Replication of the ∼30 kb-long coronavirus genome is mediated by a complex of non-structural proteins (NSP), in which NSP7 and NSP8 play a critical role in regulating the RNA-dependent RNA polymerase (RdRP) activity of NSP12. The central unit of the replication machinery is NSP12, which is responsible for the RNA-dependent RNA polymerase (RdRP) activity. In addition, NSP7 and NSP8, with molecular weights of ∼9 and ∼22 kDa, respectively, serve to promote the replication processivity of NSP12 (5,6). We report the crystal structure of the complex between NSP7 and NSP8 of SARS-CoV-2, revealing a 2:2 heterotetrameric form.

Next, we crystalized the NSP7–NSP8 complex and solved the crystal structure at 2.7 Å resolution. The crystal structure of the NSP7-NSP8 complex belongs to the space group P21, with each asymmetric unit containing two NSP7 and NSP8 molecules. Despite the fact that full-length NSP7 and NSP8 proteins were prepared for crystallization, we were only able to trace the electron density for the C-terminal domain of NSP8 spanning from residues E77 to S193, with the N-terminal portion most likely proteolytically cleaved during crystallization. On the other hand, we were able to trace the entire NSP7 molecule except for residues L83-Q84 at its C-terminus. Analysis of the structure of the NSP7–NSP8 complex reveals a 2:2 NSP7–NSP8 tetrameric complex, formed by two closely-packed NSP7–NSP8 dimers. As previously observed for the NSP7–NSP8–NSP12 complex, NSP8 is comprised of an N-terminal domain, albeit with only two α-helices traceable here, followed by a C-terminal domain formed by a four-stranded antiparallel β-sheet packed against three intervening helices. NSP7 is comprised of four α-helices, with the last one moving apart from the first three to cradle the two N-terminal helices of NSP8, resulting in a mixed six-helix bundle. Furthermore, helix α1 of NSP8 and helices α1–α2 of NSP7 pack against the counterparts of the other NSP7–NSP8 complex to form the tetrameric structure. Close inspection of the two interfaces revealed that both the dimeric and heterotetrameric association between NSP7 and NSP8 is dominated by non-polar contacts, involving all the four helices of NSP7 and helices α1 and α2 of NSP8.

>[2x]SSKMSDVKCTSVVLLSVLQQLRVESSSKLWAQCVQLHNDILLAKDTTEAFEKMVSLLSVLLSMQGAVDINKLCEEMLDNRATLQ;>AIASEFSSLPSYAAFATAQEAYEQAVANGDSEVVLKKLKKSLNVAKSEFDRDAAMQRKLEKMADQAMTQMYKQARSEDKRAKVTSAMQTMLFTMLRKLDNDALNNIINNARDGCVPLNIIPLTTAAKLMVVIPDYNTYKNTCDGTTFTYASALWEIQQVVDADSKIVQLSEISMDNSPNLAWPLIVTALRANSAVKLQ[2x]> GGGUGGCUCUACAUUUGUUGC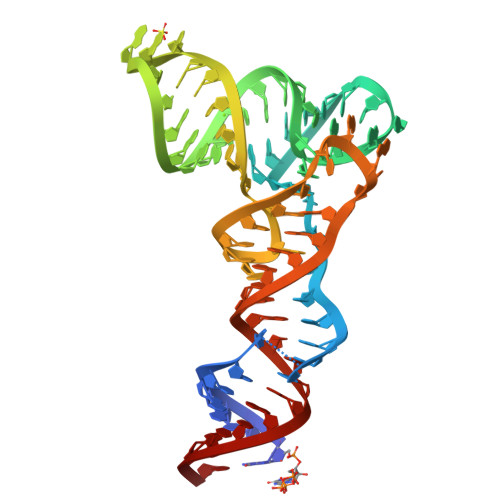GGGUUCGAGACCCGUCAGAGCGAAAGCUCUGUAGCUCAAUGGUAGAGCGGUGUAGUCACC McrBC is an antiphage defense system of Escherichia coli that specifically cleaves invading DNA that are methylated. Furthermore, upon binding of the endonuclease McrC, a higher oligomeric form—tetradecamers of 12 McrB and 2 McrC protomers—is formed. GTP hydrolysis by McrBC bound to a recognition sequence powers DNA translocation, and convergence of two such complexes on the DNA results in nucleolytic cleavage. Here we present the structure of the AAA+ domain of McrB in complex with McrC at 3.6 Å resolution using cryo-electron microscopy (cryo-EM), which reveals the coupling between the endonuclease and the motor and the mechanism of activation of the GTPase.

The complex was formed in the presence of the GTP analog 5’-guanylyl imidodiphosphate (GNP). McrBΔNC is dumbbell shaped with the two hexameric McrBΔN rings tilted with respect to each other and sandwiching an McrC dimer. Three-dimensional (3D) classification resulted in nine major classes with varying tilt angle, indicative of conformational plasticity. The two protomers of McrC in the McrBΔNC complex are related to each other by a two-fold symmetry. The dimeric interface mainly constitutes helix H9 and has a total buried surface area of ~3000 Å2. The catalytic residues, Asp244, Asp257, and Lys259, are located close to the dimeric interface and aligned along the FA interface of McrB. A particularly interesting feature of McrBΔNC is that the McrC stalk blocks the pore of the McrB ring.

>MSKTESYCLEDALNDLFIPETTIETILKRLTIKKNIILQGPPGVGKTFVARRLAYLLTGEKAPQRVNMVQFHQSYSYEDFIQGYRPNGVGFRRKDGIFYNFCQQAKEQPEKKYIFIIDEINRANLSKVFGEVMMLMEHDKRGENWSVPLTYSENDEERFYVPENVYIIGLMNTADRSLAVVDYALRRRFSFIDIEPGFDTPQFRNFLLNKKAEPSFVESLCQKMNELNQEISKEATILGKGFRIGHSYFCCGLEDGTSPDTQWLNEIVMTDIAPLLEEYFFDDPYKQQKWTNKLLGDSSGSHHHHHH[12x];>MEQPVIPVRNIYYMLTYAWGYLQEIKQANLEAIPGNNLLDILGYVLNKGVLQLSRRGLELDYNPNTEIIPGIKGRIEFAKTIRGFHLNHGKTVSTFDMLNEDTLANRIIKSTLAILIKHEKLNSTIRDEARSLYRKLPGISTLHLTPQHFSYLNGGKNTRYYKFVISVCKFIVNNSIPGQNKGHYRFYDFERNEKEMSLLYQKFLYEFCRRELTSANTTRSYLKWDASSISDQSLNLLPRMETDITIRSSEKILIVDAKYYKSIFSRRMGTEKFHSQNLYQLMNYLWSLKPENGENIGGLLIYPHVDTAVKHRYKINGFDIGLCTVNLGQEWPCIHQELLDIFDEYLK[2x]> DDKMDYDFKVKLSSERERVEDLFEYEGCKVGRGTYGHVYKAKRKDGKDDKDYALKQIEGTGISMSACREIALLRELKHPNVISLQKVFLSHADRKVWLLFDYAEHDLWHIIKFHRASKANKKPVQLPRGMVKSLLYQILDGIHYLHANWVLHRDLKPANILVMGEGPERGRVKIADMGFARLFNSPLKPLADLDPVVVTFWYRAPELLLGARHYTKAIDIWAIGCIFAELLTSEPIFHCRQEDIKTSNPYHHDQLDRIFNVMGFPADKDWEDIKKMPEHSTLMKDFRRNTYTNCSLIKYMEKHKVKPDSKAFHLLQKLLTMDPIKRITSEQAMQDPYFLEDPLPTSDVFAGCQIPYPKREFLTEEEPDDKGDKKNQQQQQGNNHTNGTGHPGNQDSSHTQGPPLKK;> DDKAMAGNFWQSSHYLQWILDKQDLLKERQKDLKFLSEEEYWKLQIFFTNVIQALGEHLKLRQQVIATATVYFKRFYARYSLKSIDPVLMAPTCVFLASKVEEFGVVSNTRLIAAATSVLKTRFSYAFPKEFP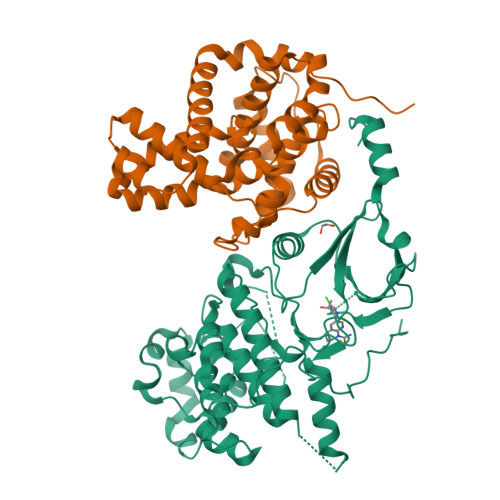YRMNHILECEFYLLELMDCCLIVYHPYRPLLQYVQDMGQEDMLLPLAWRIVNDTYRTDLCLLYPPFMIALACLHVACVVQQKDARQWFAELSVDMEKILEIIRVILKLYEQWKNFDERKEMATILSKMPKPKPPPNSEGEQGPNGSQNSSYSQS>GPAGAQDDVPPYFKTEPVRTQVHLEGNRLVLTCMAEGSWPLEFKWLHNNRELTRFSLEYRYMITSLDRTHAGFYRCIVRNRMGALLQRQTEVQVAYMGSFEEGEKRQSVNHGEAAVIRAPRISSFPRPQVTWFRDGRKIPPSSRIAITLENTLVILSTVAPDAGRYYVQAVNDKNGDNKTSQP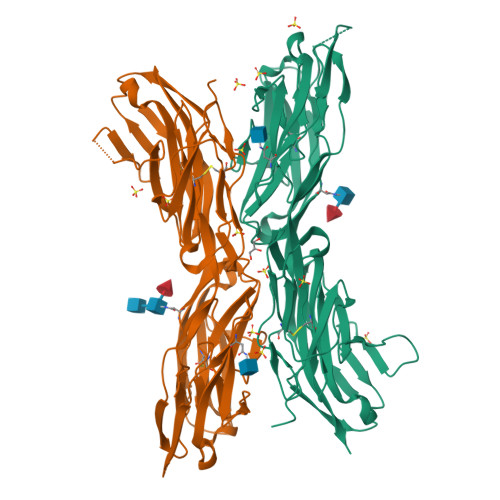ITLAVENVGGPADPIAPTIIIPPKNTSVVAGTSEVTMECVANARPLIKLHIVWKKDGAPLSSGISDYNRRLTIANPTVSDAGYYECEAMLRSSSVAPVTRGAYLSVLEPPQFVREPERHITAEMEKVVDIPCRAKGVPPPSITWYKDAALVEVGKLTRFKQRSDGGLQISGLLPDDTGMLQCFAHNAAGEAQTSTYLAVTS[2x]> GSGREEDPHEGKIWFHGKISKQEAYNLLMTVGQVSSFLVRPSDNTPGDYSLYFRTNENIQRFKISPTPNNQFMMGGRYYNSIGD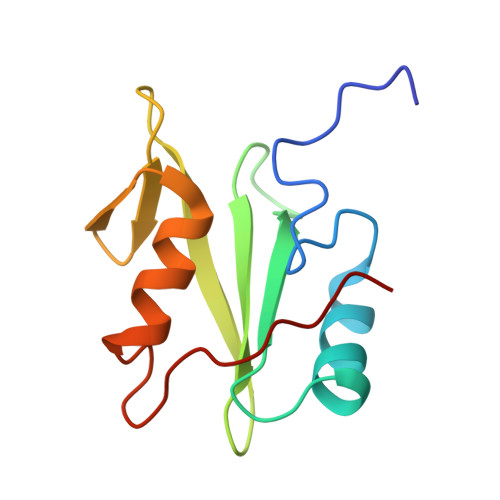IIDHYRKEQIVEGYYLKEPVPMQ> VDKRESYTKEDLLASGRGELFGAKGPQLPAPNMLMMDRVVKMTETGGNFDKGYVEAELDINPDLWFFGCHFIGDPVMPGCLGLDAMWQLVGFYLGWLGGEGKGRALGVGEVKFTGQVLPTAKKVTYRIHFKRIVNRRLIMGLADGEVLVDGRLIYTASDLKVGLFQDTSAFVDKRESYTKEDLLASGRGEL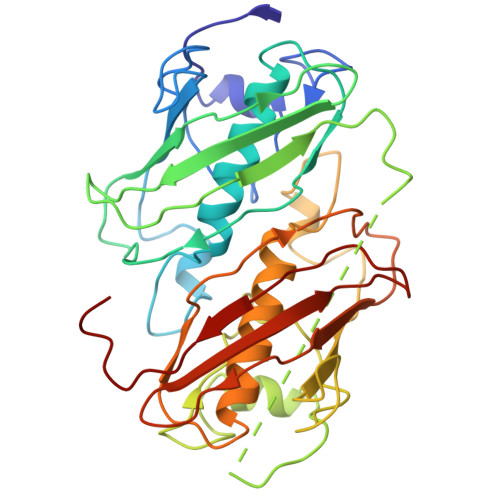FGAKGPQLPAPNMLMMDRVVKMTETGGNFDKGYVEAELDINPDLWFFGCHFIGDPVMPGCLGLDAMWQLVGFYLGWLGGEGKGRALGVGEVKFTGQVLPTAKKVTYRIHFKRIVNRRLIMGLADGEVLVDGRLIYTASDLKVGLFQDTSAF> MGAQLSKNTAGSHTTGTYATGGSSIHYTNINYYEN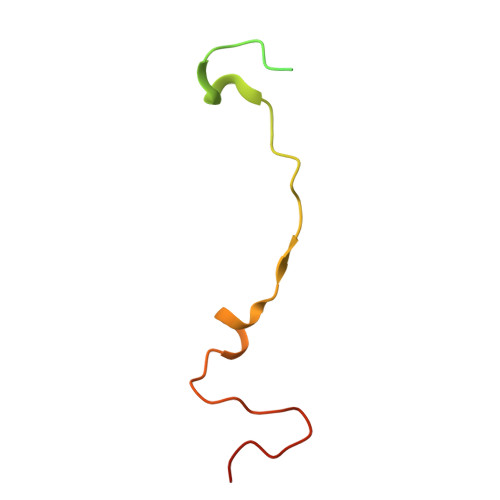AASNSLNKQDFTQDPDKFTRPVADIMKEAAVPLKSP>GSHMDYI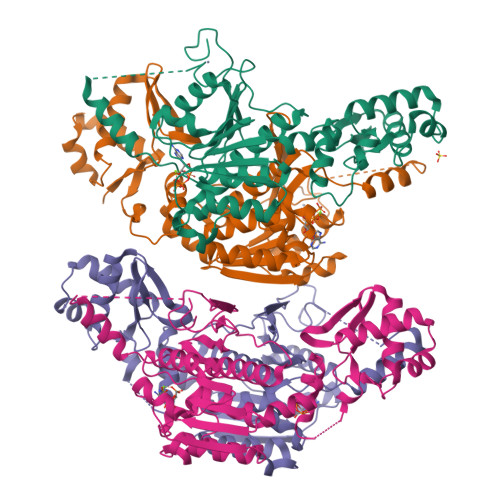LGRYVKIARYGSGGLVGGGGKEQYVENLVLWENIIKTAYCFITPSSYTAALETANIPEKDFSNCFRFLKENFFIIPGEYNNSTENNRYSRNFLHYQSYGANPVLVQDKLKNAKVVILGCGGIGNHVSVILATSGIGEIILIDNDQIENTNLTRQVLFSEDDVGKNKTEVIKRELLKRNSEISVSEIALNINDYTDLHKVPEADIWVVSADHPFNLINWVNKYCVRANQPYINAGYVNDIAVFGPLYVPGKTGCYECQKVVADLYGSEKENIDHKIKLINSRFKPATFAPVNNVAAALCAADVIKFIGKYSEPLSLNKRIGIWSDEIKIHSQNMGRSPVCSVCGNRM[4x]> MAAKSYNIPELDKKLADRRYHLSDTNPEFTQKILKTSRTIANMCYQCGTCTGSCPSAP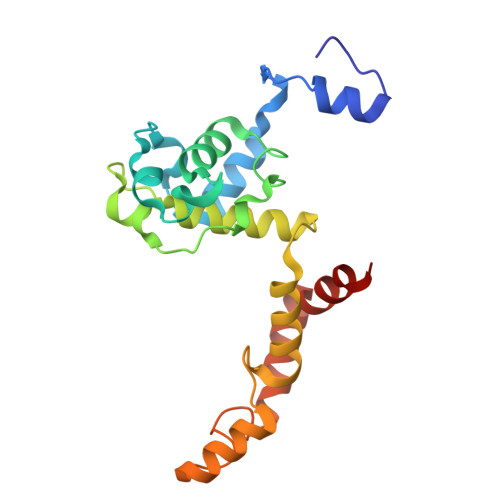RSSYRIRLFMRRCVLGLENEALTDPDLWLCTTCYSCTDRCPRDIAPTDVIMAMRNLAFKRDIVPKNFLQTVQLIYNSGHGVPNNDVNRAARTKLGLPADPPTTHSYPEFVKGIQKIIDHYELKENADRILKGD> MMELIRIAMKKDLENDNSLMNKWATVAGLKNPNPLYDFLNHDGKTFNEFSSIVNIVKSQYPDREYELMKDYCLNLDVKTKAARSALEYADANMFFEIEDVLIDSMISCSNMKSKEYGKVYKIHRELSNSVITEFEAVKRLGKLNIKTPEMNSFSRLLLLYHYLSTGNFSPMAQLIKQIDLSEISENMYIRNTYQTRVHVLMSNIKLNENSLEECREYSKKALESTNILRFQVFSYLTIGNSLLFSNYELAQENFLKGLSISVQNENYNMIFQQALCFLNNVWRKENKWINFESDSIMDLQEQAHCFINFNENSKAKEVLDKLDLLVHNDNELAMHYYLKGRLEQNKACFYSSIEYFKKSNDKFLIRLPLLELQKMGENQKLLELLLLLEH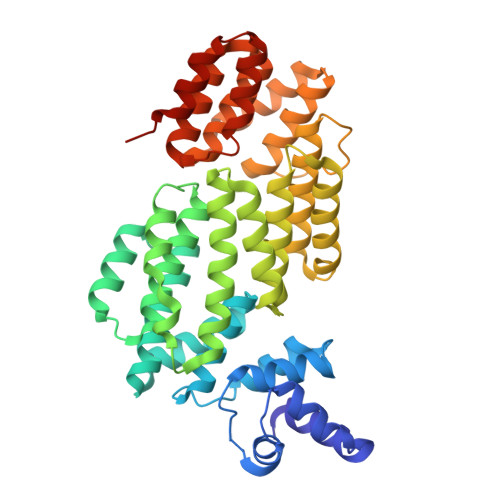HHHHH>MKDLVDTTEMYLRTIYELEEEGVTPLRARIAERLEQSGPTVSQTVARMERDGLVVVASDRSLQMTPTGRTLATAVMRKHRLAERLLTDIIGLDINKVHDEACRWEHVMSDEVERRLVKVLKDVSRSPFGNPIPGLDELGVGNSDAAAPGTRV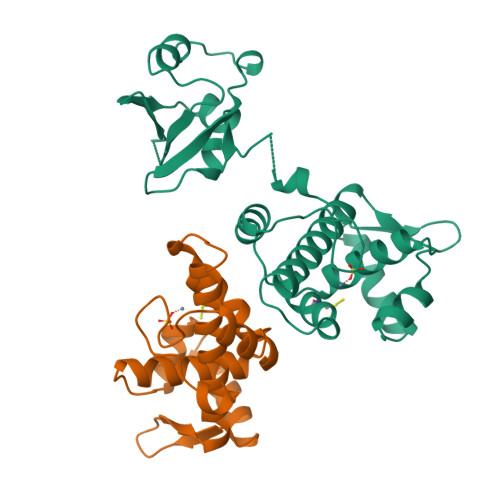IDAATSMPRKVRIVQINEIFQVETDQFTQLLDADIRVGSEVEIVDRDGHITLSHNGKDVELLDDLAHTIRIEEL[2x]> KMAKLYMVSDASGSMRVTVVAEENPFSMAMLLSEECFILDHGAAKQIFVWKGKDANPQERKAAMKTAEEFLQQMNYSKNTQIQVLPEGGETPIFKQFF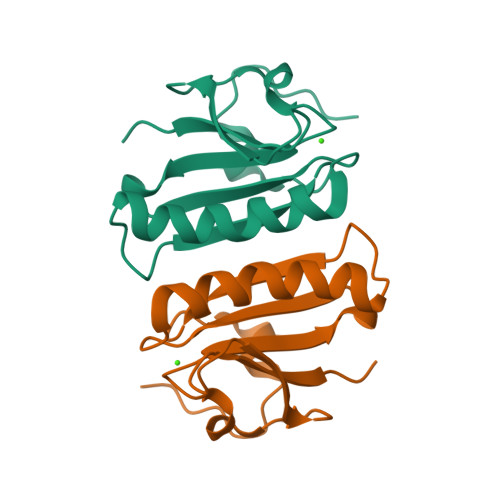KDWRDK N-{4-methyl-3-[8-methyl-7-oxo-2-(phenylamino)-7,8-dihydropyrido[2,3-d]pyrimidin-6-yl]phenyl}-3-(trifluoromethyl)benzamide 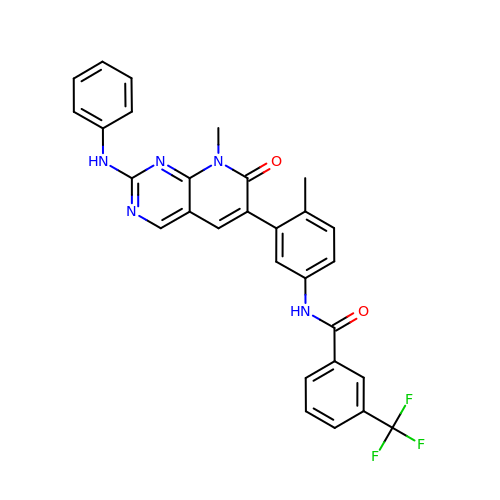| C29 H22 F3 N5 O2 | IMLLFFIWQIAPHC-UHFFFAOYSA-N>[4x]MEKKVLLTGFDPFGGETVNPSWEA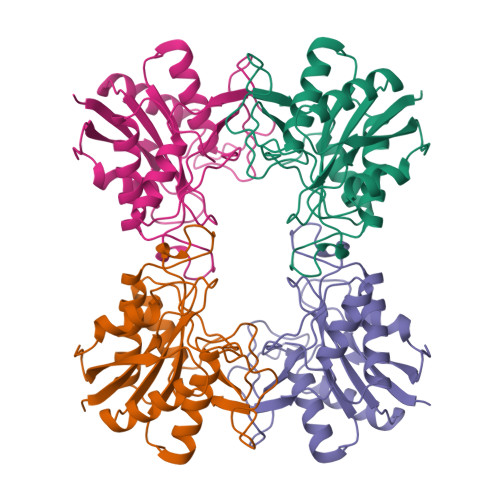VKRLNGAAEGPASIVSEQVPTVFYKSLAVLREAIKKHQPDIIICVGQAGGRMQITPERVAINLNEARIPDNEGNQPVGEDISQGGPAAYWTGLPIKRIVEEIKKEGIPAAVSYTAGTFVCNHLFYGLMDEISRHHPHIRGGFIHIPYIPEQTLQKSAPSLSLDHITKALKIAAVTAAVHEDDIETGGGELH> SADAQSFLNRVCGVSAARLTPCGTGTSTDVVYRAFDIYNDKVAGFAKFLKTNCCRFQEKDEDDNLIDSYFVV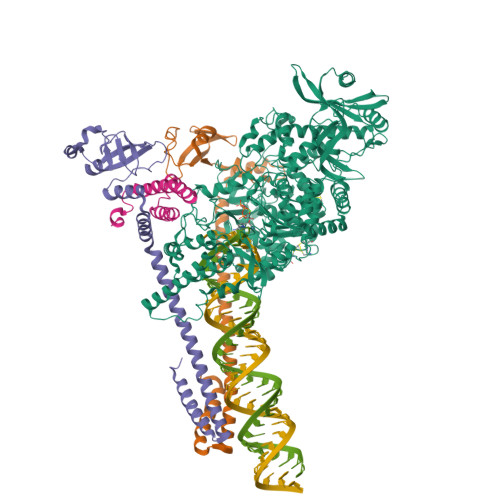KRHTFSNYQHEETIYNLLKDCPAVAKHDFFKFRIDGDMVPHISRQRLTKYTMADLVYALRHFDEGNCDTLKEILVTYNCCDDDYFNKKDWYDFVENPDILRVYANLGERVRQALLKTVQFCDAMRNAGIVGVLTLDNQDLNGNWYDFGDFIQTTPGSGVPVVDSYYSLLMPILTLTRALTAESHVDTDLTKPYIKWDLLKYDFTEERLKLFDRYFKYWDQTYHPNCVNCLDDRCILHCANFNVLFSTVFPPTSFGPLVRKIFVDGVPFVVSTGYHFRELGVVHNQDVNLHSSRLSFKELLVYAADPAMHAASGNLLLDKRTTCFSVAALTNNVAFQTVKPGNFNKDFYDFAVSKGFFKEGSSVELKHFFFAQDGNAAISDYDYYRYNLPTMCDIRQLLFVVEVVDKYFDCYDGGCINANQVIVNNLDKSAGFPFNKWGKARLYYDSMSYEDQDALFAYTKRNVIPTITQMNLKYAISAKNRARTVAGVSICSTMTNRQFHQKLLKSIAATRGATVVIGTSKFYGGWHNMLKTVYSDVENPHLMGWDYPKCDRAMPNMLRIMASLVLARKHTTCCSLSHRFYRLANECAQVLSEMVMCGGSLYVKPGGTSSGDATTAYANSVFNICQAVTANVNALLSTDGNKIADKYVRNLQHRLYECLYRNRDVDTDFVNEFYAYLRKHFSMMILSDDAVVCFNSTYASQGLVASIKNFKSVLYYQNNVFMSEAKCWTETDLTKGPHEFCSQHTMLVKQGDDYVYLPYPDPSRILGAGCFVDDIVKTDGTLMIERFVSLAIDAYPLTKHPNQEYADVFHLYLQYIRKLHDELTGHMLDMYSVMLTNDNTSRYWEPEFYEAMYTPHTVLQ;>AIASEFSSLPSYAAFATAQEAYEQAVANGDSEVVLKKLKKSLNVAKSEFDRDAAMQRKLEKMADQAMTQMYKQARSEDKRAKVTSAMQTMLFTMLRKLDNDALNNIINNARDGCVPLNIIPLTTAAKLMVVIPDYNTYKNTCDGTTFTYASALWEIQQVVDADSKIVQLSEISMDNSPNLAWPLIVTALRANSAVKLQ[2x];> VACTKEVHMSKMSDVKCTSVVLLSVLQQLRVESSSKLWAQCVQLHNDILLAKDTTEAFEKMVSLLSVLLSMQGAVDINKLCEEMLDNRATLQ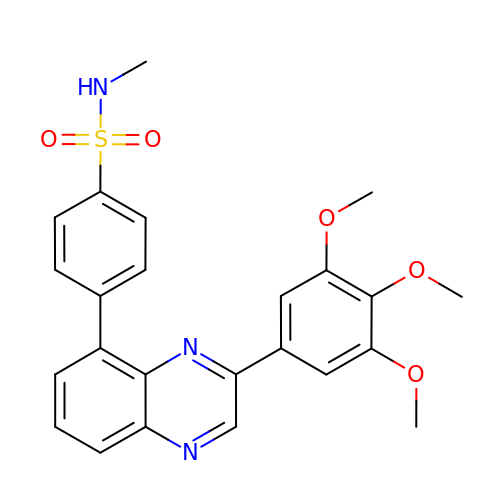N-methyl-4-[3-(3,4,5-trimethoxyphenyl)quinoxalin-5-yl]benzenesulfonamide | C24 H23 N3 O5 S | LYSCAOWDVVWGQK-UHFFFAOYSA-N>MNVEEMKKIAAKEALKFIEDDMVIGLGTGSTTAYFIKLLGEKLKRGEISDIVGVPTSYQAKLLAIEHDIPIASLDQVDAIDVAVDGADEVDPNLNLIKGRGAALTMEKIIEYRAGTFIVLVDERKLVDYLCQKMPVPIEVIPQAWKAIIEEL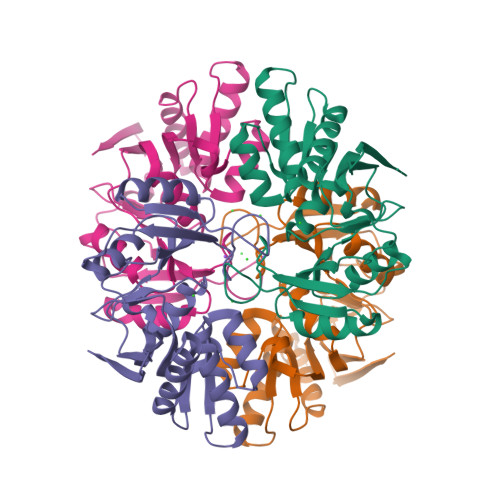SIFNAKAELRMGVNKDGPVITDNGNFIIDAKFPRIDDPLDMEIELNTIPGVIENGIFADIADIVIVGTREGVKKLER[4x]> MLRDLFDRAVVLSHYIANLSSEMFSEFDKRYTHGRGFITKAINSCHTSSLATPEDKEQAQQMNQKDFLSLIVSILRSWNEPLYHLVTEVRGMQEAPEAILSKAVEIEEQTKRLLERMELIVSQVHPETKENEIYPVWSGLPSLQMADEESRLSAYYNLLHCLRRDSHKIDNYLKLLKCRIIHNNNC;> MLPPGKPEIFK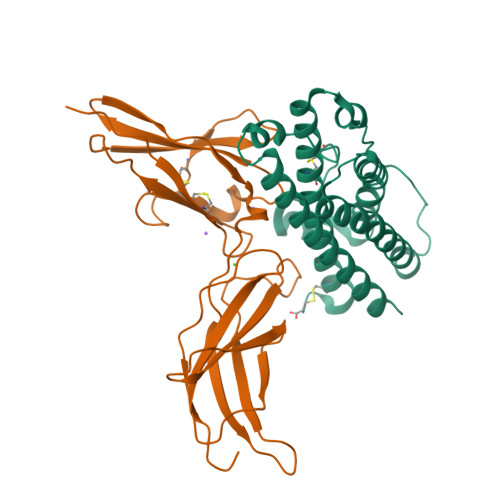CRSPNKETFTCWWRPGTDGGLPTNYSLTYHREGETLMHECPDYITGGPNSCHFGKQYTSMWRTYIMMVNATNQMGSSFSDELYVDVTYIVQPDPPLELAVEVKQPEDRKPYLWIKWSPPTLIDLKTGWFTLLYEIRLKPEKAAEWEIHFAGQQTEFKILSLHPGQKYLVQVRCKPDHGYWSAWSPATFIQIPSDFTMND> MAHHHHHHMSDEDHDFSHQGGGDNASKTYPLAAGALKKGGYVCINGRPCKVIDL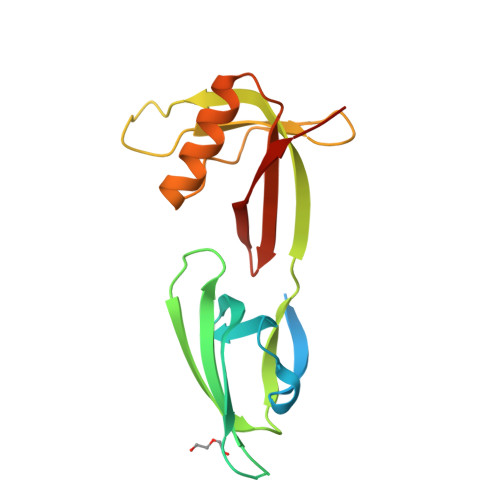SVSKTGKHGHAKVSIVATDIFTGNRLEDQAPSTHNVEVPFVKTYTYSVLDIQANEDPSLPAHLSLMDDEGESREDLDMPPDPALATQIKEQFDSGKDVLVVVVSAMGTEQVLQTKNAAEK> MDKSSIANKIEAYLGAKSDDSKIDQSLKADPSEVQYYGSGGDGYYLRKNICKITVNHSDSGTNDPCDRIPPPYGDNDQWKCAIILSKVSEKPENVFVPPRRQRMCINNLEKLNVDKIRDKHAFLADVLLTARNEGERIVQNHPDTNSSNVCNALERSFADIADIIRGTDLWKGTNSNLEQNLKQMFAKIRENDKVLQDKYPKDQNYRKLREDWWNANRQKVWEVITCGARSNDLLIKRGWRTSGKSNGDNKLELCRKCGHYEEKVPTKLDYVPQFLRWLTEWIEDFYREKQNLIDDMERHREECTSEDHKSKEGTSYCSTCKDKCKKYCECVKKWKSEWENQKNKYTELYQQNKNETSQKNTSRYDDYVKDFFKKLEANYSSLENYIKGDPYFAEYATKLSFILNSSDANNPSEKIQKNNDEVCNCNESGIASVEQEQISDPSSNKTCITHSSIKANKKKVCKHVKLGVRENDKDLRVCVIEHTSLSGVENCCCQDFLRILQENCSDNKSGSSSNGSCNNKNQEACEKNLEKVLASLTNCYKCDKCKSEQSKKNNKNWIWKKSSGKEGGLQKEYANTIGLPPRTQSLCLVVCLDEKGKKTQELKNIRTNSELLKEWIIAAFHEGKNLKPSHEKKNDDNGKKLCKALEYSFADYGDLIKGTSIWDNEYTKDLELNLQKIFGKLFRKYIKKNNTAEQDTSYSSLDELRESWWNTNKKYIWLAMKHGAGMNSTTCCGDGSVTGSGSSCDDIPTIDLIPQYLRFLQEWVEHFCKQRQEKVKPVIENCKSCKESGGTCNGECKTECKNKCEVYKKFIEDCKGGDGTAGSSWVKRWDQIYKRYSKYIEDAKRNRKAGTKNCGPSSTTNAAENKCVQSDIDSFFKHLIDIGLTTPSSYLSIVLDDNICGADKAPWTTYTTYTTTEKCNKETDKSKLQQCNTAVVVNVPSPLGNTPHGYKYACQCKIPTNEETCDDRKEYMNQWSCGSARTMKRGYKNDNYELCKYNGVDVKPTTVRSNSSKLDDKDVTFFNLFEQWNKEIQYQIEQYMTNTKISCNNEKNVLSRVSDEAAQPKFSDNERDRNSITHEDKNCKEKCKCYSLWIEKINDQWDKQKDNYNKFQRKQIYDANKGSQNKKVVSLSNFLFFSCWEEYIQKYFNGDWSKIKNIGSDTFEFLIKKCGNDSGDGETIFSEKLNNAEKKCKENESTNNKMKSSETSCDCSEPIYIRGCQPKIYDGKIFPGKGGEKQWICKDTIIHGDTNGACIPPRTQNLCVGELWDKRYGGRSNIKNDTKESLKQKIKNAIQKETELLYEYHDKGTAIISRNPMKGQKEKEEKNNDSNGLPKGFCHAVQRSFIDYKNMILGTSVNIYEYIGKLQEDIKKIIEKGTTKQNGKTVGSGAENVNAWWKGIEGEMWDAVRCAITKINKKQKKNGTFSIDECGIFPPTGNDEDQSVSWFKEWSEQFCIERLQYEKNIRDACTNNGQGDKIQGDCKRKCEEYKKYISEKKQEWDKQKTKYENKYVGKSASDLLKENYPECISANFDFIFNDNIEYKTYYPYGDYSSICSCEQVKYYEYNNAEKKNNKSLCHEKGNDRTWSKKYIKKLENGRTLEGVYVPPRRQQLCLYELFPIIIKNKNDITNAKKELLETLQIVAEREAYYLWKQYHAHNDTTYLAHKKACCAIRGSFYDLEDIIKGNDLVHDEYTKYIDSKLNEIFDSSNKNDIETKRARTDWWENEAIAVPNITGANKSDPKTIRQLVWDAMQSGVRKAIDEEKEKKKPNENFPPCMGVQHIGIAKPQFIRWLEEWTNEFCEKYTKYFEDMKSNCNLRKGADDCDDNSNIECKKACANYTNWLNPKRIEWNGMSNYYNKIYRKSNKESEDGKDYSMIMEPTVIDYLNKRCNGEINGNYICCSCKNIGENSTSGTVNKKLQKKETQCEDNKGPLDLMNKVLNKMDPKYSEHKMKCTEVYLEHVEEQLKEIDNAIKDYKLYPLDRCFDDKSKMKVCDLIGDAIGCKHKTKLDELDEWNDVDMRDPYNKYKGVLIPPRRRQLCFSRIVRGPANLRNLKEFKEEILKGAQSEGKFLGNYYNEDKDKEKALEAMKNSFYDYEYIIKGSDMLTNIQFKDIKRKLDRLLEKETNNTEKVDDWWETNKKSIWNAMLCGYKKSGNKIIDPSWCTIPTTETPPQFLRWIKEWGTNVCIQKEEHKEYVKSKCSNVTNLGAQESESKNCTSEIKKYQEWSRKRSIQWEAISEGYKKYKGMDEFKNTFKNIKEPDANEPNANEYLKKHCSKCPCGFNDMQEITKYTNIGNEAFKQIKEQVDIPAELEDVIYRLKHHEYDKGNDYICNKYKNINVNMKKNNDDTWTDLVKNSSDINKGVLLPPRRKNLFLKIDESDICKYKRDPKLFKDFIYSSAISEVERLKKVYGEAKTKVVHAMKYSFADIGSIIKGDDMMENNSSDKIGKILGDGVGQNEKRKKWWDMNKYHIWESMLCGYKHAYGNISENDRKMLDIPNNDDEHQFLRWFQEWTENFCTKRNELYENMVTACNSAKCNTSNGSVDKKECTEACKNYSNFILIKKKEYQSLNSQYDMNYKETKAEKKESPEYFKDKCNGECSCLSEYFKDETRWKNPYETLDDTEVKNN

VAR2CSA encoded by a subfamily of var genes from Plasmodium falciparum (P. falciparum) named as var2csa, plays a vital role in the cytoadherence of infected erythrocytes to the placenta. In this study, the VAR2CSA ectodomain from P. falciparum strain 3D7 (~306 kDa, containing six Duffy-binding-like (DBL) domains, N-terminal sequence (NTS), and multiple inter-domains (IDs))8 was recombinantly expressed and purified using the Sf9 insect cell secretory system. The cryo-EM structures of VAR2CSA ectodomain and its complex with CSA were determined at a resolution of 3.6 Å and 3.4 Å, respectively. In line with the previously proposed model, our structures showed that the core region is well-defined and covers NTS, DBL1X, DBL2X, ID2a, ID2b, DBL3X, ID3, and DBL4ε.

Compared with the apo structure, the densities of the wing region in the complex were significantly improved, making it feasible for the flexible fitting of both DBL5ε and DBL6ε. Intriguingly, a highly basic pocket formed by DBL2X, DBL1X, NTS, and DBL4ɛ has been identified to accommodate a dodecasaccharide with six sulfated disaccharide repeats from CSA, which fitted well into the density map. Moreover, 16 residues were identified to be responsible for the direct interaction with 10/12 monosaccharides, except for the 6th and 11th units of CSA dodecasaccharide. Among them, there are nine, four, and three residues derived from DBL2X, DBL4ɛ, and NTS, respectively. Furthermore, the nine residues of DBL2X were shown to interact directly with 7/10 monosaccharide units and thus may account for the major contribution to CSA binding. Owing to its high resolution and potential high stability in the core center, DBL4ɛ was used as an immobilized reference for the structural alignment between the VAR2CSA-CSA and VAR2CSA ectodomain. Interestingly, a significant conformational change in the core region was observed. Firstly, the DBL1X moves closer to DBL4ɛ at more than 3.2 Å (ranging from 3.2 Å to 4.4 Å) for multi-helixes to facilitate NTS interaction with CSA and close the pocket. Secondly, there was a 1.8 Å outward bend for the key CSA binding helix of DBL2X in the deep pocket. Lastly, the rest of DBL2X moved about 2 Å inward to shrink the pocket.> GPMSEKIEGIIDDLLNLEENAHGIAIIGKDGKIITQTENWNISND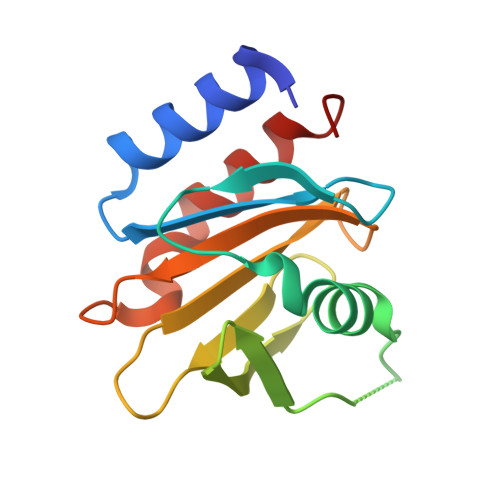LDKLNEFLNEKLALGKKGITSLSIQGIKYMIVENTEERKIGTNITGKGHVVICPIPIGGTGALITYVNPRAGPRDVLFNVQEYAKKLTDLI>GSMTTVMNDKHPTPDPAEDNAFFPSAYSLSQFTASKSDLSGAHYPTPYQGGRWKILVVGADERYLMMDNGTFFSTGNHPVATLLPMYHLDKAGFSFDIATLSGNPVKFEWWAMPREDQEVNGLYSKYQSSFRQPLKLSDVIETALGEDSDYIGVFIPGGHGALMGLPDSQEVKAVLQWAMKQNKF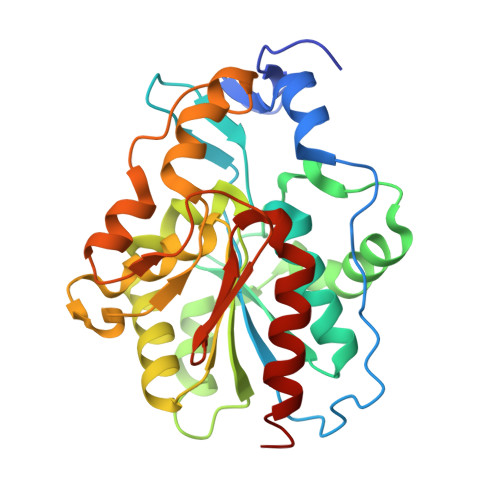IISLCHGPAAFLAVGDDPLFAGYKIVAFPDEMDAQTPSIGYMPGHLTWKFGEQLQAIGFELLNTGISGQVFQDRKMLTGDSPLAGNALGQLAAKALLAEVEQK[6x]> MSEEEVDKVYRRLNQEVEKSGYHLNPDVEFTKEL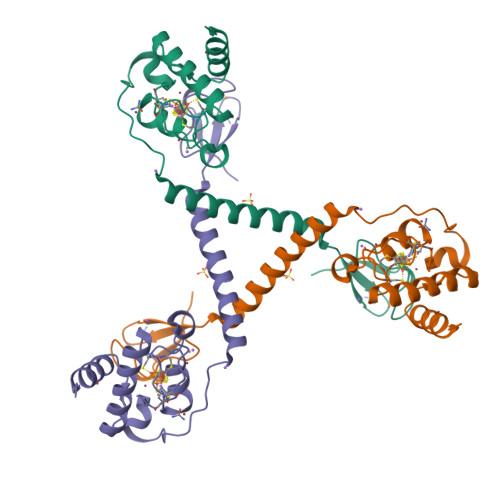VRGLLANERRYGYWSCPCRLSADNKEEDLDIICPCYYRDPDLNDYGACYCALYVSDEVIRGEKEVESIPERRPPREKREAIRAEEASRAEMMETMEFTGKLSKPVWRCKVCGYLCAMDEAPGVCPICKARKERFERFMH>[2x]MSDSKPRDVQVLPIATNTKVLRARSWSRLRFEIEYALERGTTSNSYVIEGDKTAIIDPPVESFMKIYLEALQQTVNLKKLDYVILGHFSPNRIPTFKALLELAPQITFVCSLPAAGDLRAAFPDDNLNILPMRGKETLDLGKGHVLKFLPIPSPRWPAGLCTYDVQTQILYTDKIFGAHICGDDVFDDNWESFKED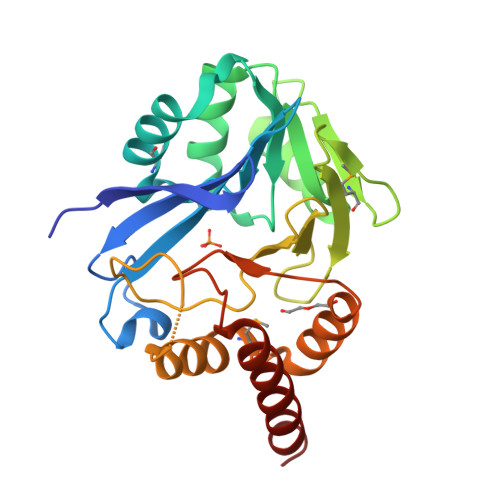QRYYFNCLMAPHAIHVEAALEKISDLQVRLYAVGHGPLVRTSLIALTQAYADWSKAQKLEHHHHHH> MPAVDKLLLEEALQDSPQTRSLLSVFEEDAGTLTDYTNQLLQAMQRVYGAQNEMCLATQQLSKQL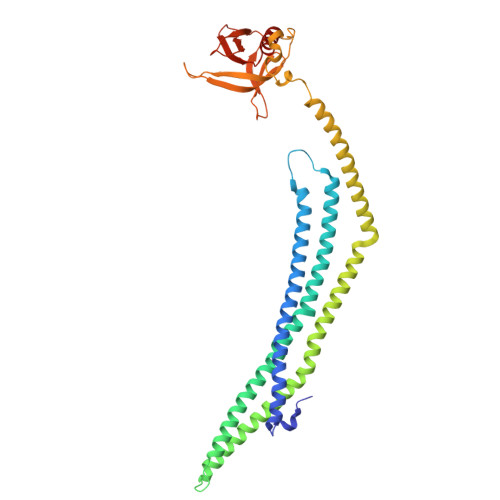LAYEKQNFALGKGDEEVISTLHYFSKVVDELNLLHTELAKQLADTMVLPIIQFREKDLTEVSTLKDLFGLASNEHDLSMAKYSRLPKKKENEKVKTEVGKEVAAARRKQHLSSLQYYCALNALQYRKQMAMMEPMIGFAHGQINFFKKGAEMFSKRMDSFLSSVADMVQSIQVELEAEAEKMRVSQQELLSVDESVYTPDSDVAAPQINRNLIQKAGYLNLRNKTGLVTTTWERLYFFTQGGNLMCQPRGAVAGGLIQDLDNCSVMAVDCEDRRYCFQITTPNGKSGIILQAESRKENEEWICAINNISR> 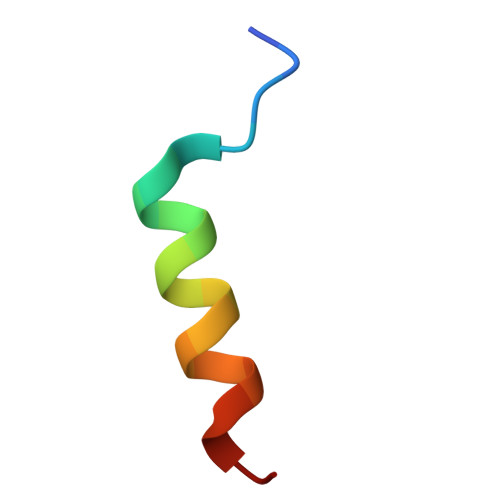AAAAAAAAAAAAAAAAAAAA>[2x]MAISLATKAATDALKVNRAPVGVEPQEVHKWLQSFNWDFKENRTKYPTKYHMANETKEQFKVIAKEYARMEAAKDERQFGTLLDGLTRLGAGNKVHPRWGETMKVISNFLEVGEYNAIAASAMLWDSATAAEQKNGYLAQVLDEIRHTHQCAFINHYYSKHYHDPAGHNDARRTRAIGPLWKGMKRVFADGFISGDAVECSVNLQLVGEACFTNPLIVAVTEWASANGDEITPTVFLSVETDELRHMANGYQTVVSIANDPASAKFLNTDLNNAFWTQQKYFTPVLGYLFEYGSKFKVEPWVKTWNRWVYEDWGGIWIGRLGKYGVESPASLRDAKRDAYWAHHDLALAAYAMWPLGFARLALPDEEDQAWFEANYPGWADHYGKIFNEWKKLGYEDPKSGFIPYQWLLANGHDVYIDRVSQVPFIPSLAKGTGS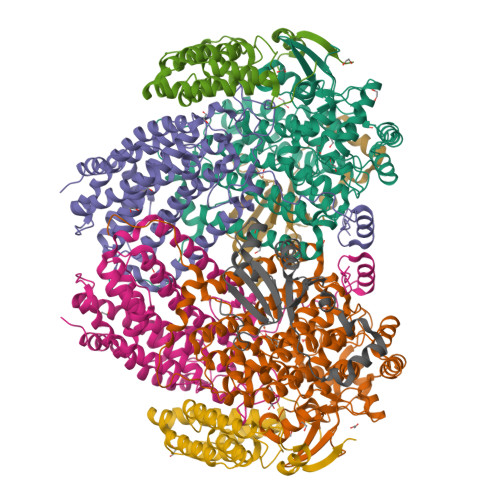LRVHEFNGKKHSLTDDWGERQWLIEPERYECHNVFEQYEGRELSEVIAEGHGVRSDGKTLIAQPHTRGDNLWTLEDIKRAGCVFPDPLAKF;>[2x]MSQPQSSQVTKRGLTDPERAAIIAAAVPDHALDTQRKYHYFIQPRWKRLSEYEQLSCYAQPNPDWIAGGLDWGDWTQKFHGGRPSWGNESTELRTTDWYRHRDPARRWHHPYVKDKSEEARYTQRFLAAYSSEGSIRTIDPYWRDEILNKYFGALLYSEYGLFNAHSSVGRDCLSDTIRQTAVFAALDKVDNAQMIQMERLFIAKLVPGFDASTDVPKKIWTTDPIYSGARATVQEIWQGVQDWNEILWAGHAVYDATFGQFARREFFQRLATVYGDTLTPFFTAQSQTYFQTTRGAIDDLFVYCLANDSEFGAHNRTFLNAWTEHYLASSVAALKDFVGLYAKVEKVAGATDRAGVSEALQRVFGDWKIDYADKIGFRVDVDQKVDAVLAGYKN;>MAKREPIHDNSIRTEWEAKIAKLTSVDQATKFIQDFRLAYTSPFRKSYDIDVDYQYIERKIEEKLSVLKTEKLPVADLITKATTGEDAAAVEATWIAKIKAAKSKYEAERIHIEFRQLYKPPVLPVNVFLRTDAALGTVLMEIRNTDYYGTPLEGLRKERGVKVLHLQA[2x];>[2x]MSSAHNAYNAGIMQKTGKAFADEFFAEENQVVHESNAVVLVLMKSDEIDAIIEDIVLKGGKAKNPSIVVEDKAGFWWIKADGAIEIDAAEAGELLGKPFSVYDLLINVSSTVGRAYTLGTKFTITSELMGLDRALTDI> MHHHHHHGENLYFQGSAPYASLTEIEHLVQSVCKSYRETCQLRLEDLLRQRSNIFSREEVTGYQRKSMWEMWERCAHHLTEAIQYVVEFAKRLSGFMELCQNDQIVLLKAGAM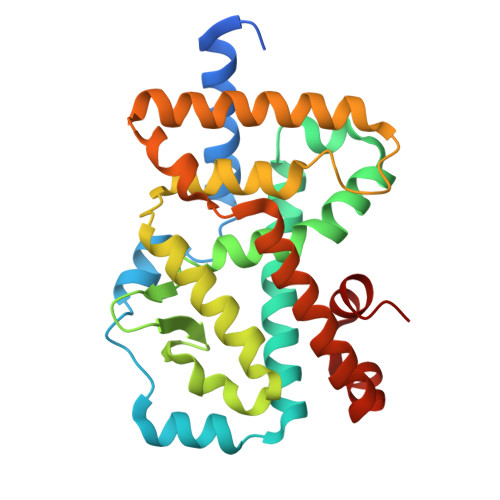EVVLVRMCRAYNADNRTVFFEGKYGGMELFRALGCSELISSIFDFSHSLSALHFSEDEIALYTALVLINAHRPGLQEKRKVEQLQYNLELAFHHHLCKTHRQSILAKLPPKGKLRSLCSQHVERLQIFQHLHPIVVQAAFPPLYKELFSTE Galectins are a family of proteins with some specificity for β-galactoside binding at their carbohydrate-recognition domain (CRD). Tandem-repeat-type galectins, like Gal-8, contain two distinct CRDs that are covalently connected via a peptide linker. In the present study, we used different conditions to crystallize the Gal-8 N-terminal CRD with its linker, and five structures could be solved. The N-terminal CRD prefers sulfated and sialylated glycans, whereas the C-terminal CRD prefers blood group A/B. In particular, the N-terminal CRD strongly binds to sulfated and sialylated glycans.

The best structure, structure 1, allowed 152 residues (Asn7 to Gln158) to be identified with 1.08 Å resolution. This is the best resolution for the Gal-8 N CRD available to date. Electron density of the first four residues in the linker region (Ser154 to Gln158) was clear, indicating that this part of linker forms stable secondary structure under conditions of our crystallization. In structure 1, four residues (Asn7, Gln9, Asp156, and Gln158) were seen to interact with each other via ionic interactions and hydrogen bonds. Surprisingly, crystal structure 1 made using the first condition has space group P212121, and not C2, and the carbohydrate binding site binds glycerol and not lactose. This structure was solved with the crystal being soaked in 20% (v/v) glycerol for approximately 1 min prior to data collection. In structure 1, glycerol was found to replace lactose in the carbohydrate binding site. In our crystal structure, the C and O atoms of glycerol occupy the same positions as C4, C5, C6 and O1, O4, O6 atoms of galactose in the lactose-bound structure. Interestingly, glycerol was found to substitute lactose at the carbohydrate binding site in 1.08 Å structure, however, because the hemagglutination assay showed that glycerol did not inhibit Gal-8 N-mediated agglutination, this ligand could not be physiologically relevant.

> NLQNIIYNPVIPFVGTIPDQLDPGTLIVIRGHVPSDADRFQVDLQNGSSMKPRADVAFHFNPRFKRAGCIVCNTLINEKWGREEITYDTPFKREKSFEIVIMVLKDKFQVAVNGKHTLLYGHRIGPEKIDTLGIYGKVNIHSIGFSFSSDLQ>[8x]GKEWQENKSWNAHFTEHKSQGVVVLWNENKQQGFTNNLKRANQAFLPASTFKIPNSLIALDLGVVKDEHQVFKWDGQTRDI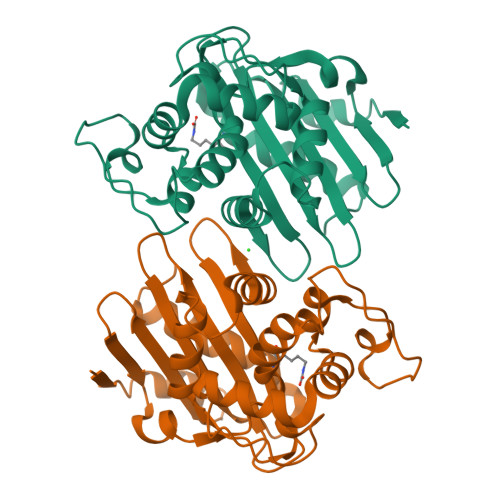ATWNRDHNLITAMKYSVVPVYQEFARQIGEARMSKMLHAFDYGNEDISGNVDSFWLDGGIRISATEQISFLRKLYHNKLHVSERSQAIVKQAMLTEANGDYIIRAKTGYSTRIEPKIGWWVGWVELDDNVWFFAMNMDMPTSDGLGLRQAITKEVLKQEKIIP>GAMGNKEQKNNNNVKEVSDSVQEDGLNDLYNNQEKQKSFTKNFGERKYEDLINPIEPIIPSESPKNKANIPNISIAHTEKKETKKENLIPSTNEEKEADAAIKYLEENILKNSKFSELIREVRVIKDEYALIKADLYDVIGKINNKKTSLMENPKNNRDKINKLTQLLQNNLKIDSELEQLINMIDMAENEISSAAFFFDNAQKRLKESIIKRLESKNNRSYALKLSRQALSDARSALSNLESFASKRIEPMVRKEEIKELIKHAKTVLESLNKK[2x]

We determined the crystal structure of a previously uncharacterized B. burgdorferi outer surface protein BBK01, known to belong to the paralogous gene family 12 (PFam12) as one of its five members. In a recent article studying the antigenicity and immunogenicity of PFam12 members, it was suggested to rename the proteins as family twelve lipoproteins (Ftl) FtlA (BBK01), FtlB (BBG01), FtlC (BBH37), and FtlD (BBJ08). Structural analysis of BBK01 revealed similarity to the coiled coil domain of structural maintenance of chromosomes (SMC) protein family members, while functional studies indicated that all PFam12 members are non-specific DNA-binding proteins. In the current study we focused on the paralogous gene family 12 (PFam12), which contains five members (BB0844, BBG01, BBH37, BBJ08, and BBK01) that do not demonstrate meaningful sequence identity with proteins from any other organism which would allow us to judge the functions of these proteins. It is known that PFam12 members are surface-exposed and highly immunogenic lipoproteins that are upregulated as the tick starts the blood meal.

The protein crystals of FtlA diffracted to 2.7 Å resolution, and the crystal structure was determined by a single-wavelength anomalous diffraction (SAD) technique. The space group was C2 with two protomers per asymmetric unit. However, in the crystal structure of FtlA, only residues 110–297 were built in the final model, as electron density was not observed for N-terminal residues 28–109. The assumption that approximately the first 80 N-terminal residues in FtlA are disordered was approved by the AlphaFold predicted model; therefore, the flexible nature of the N-terminal residues can explain their absence in the crystal structure of FtlA. The overall monomer structure of FtlA consists of two comparatively short α-helices, αA and αB, and a 120 residue long helix αC, which are connected by short loop regions. In the protein crystal, FtlA forms a homodimer where the αC from one of the monomers interacts with the same α-helix in the other monomer by forming an antiparallel coiled coil structure of approximately 180 Ǻ in length. As the dimer interface is made by residues found on all three α-helices by interacting with the equivalent residues on the other monomer, the homodimer forms a massive 7950 Ǻ2 buried surface area as detected from PISA assembly analysis and involves more than 50 residues. As judged from the crystal structure of FtlA and taking into account the conserved residues of the PFam12 members, the potential DNA-binding site in the PFam12 proteins might be located in the middle of the dimer, along residues Arg242, Arg235, and Lys118 or the distal ends of the dimer where conserved residues Lys281 and Lys182 are located. This assumption is supported by the electrostatic surface potential map, which shows a distinctive positive charge at the middle segment of FtlA and at both ends of the dimer.(2S)-2-(2-oxidanylidenepyrrolidin-1-yl)butanamide 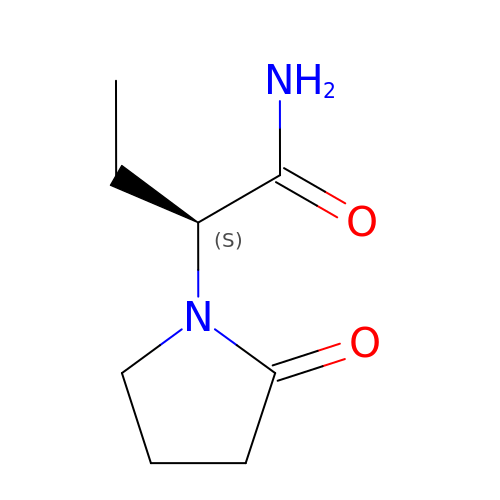| C8 H14 N2 O2 | HPHUVLMMVZITSG-LURJTMIESA-N>GDEEEKHLRDMMEIVIKLFMTGDWDAFHEMADPDVKFQVDVGDKHIHRHGREEVVEELIRLLEHWRVRNIRIHDIKLIGDKLVVEGRWETSYGDKSHDEDVE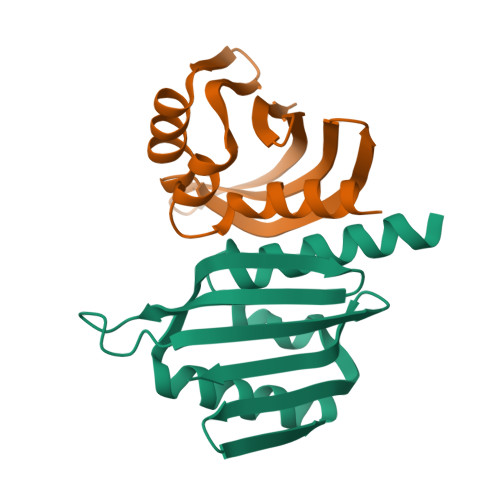LIVIVVDGKIKKVRIIIR[2x]> GSHMATFPELLRPLKLGRYTLRNRIIMAPLTRCQATEDGHVPRTESMLKYYEDRASAGLIIAEATMVQPNYTGFLTEPGIYSDAQIEEWRKIVDAVHKKGGLIFLQLIHAGRAGIPEKILQQPKSDQDPLAGRLLAASAIPIKDHRIPAYFAASGEKETYGVPEELTDDEVRNGIIPLFVEGAKNAIFKAGFDGVEIHGANGYLLDAFFRESSNKRQSGPYAGTTIDTRCQLIYDVTKSVCDAVGSDRVGLRISPLNGVHGMIDSNPEALTKHLCKKIEPLSLAYLHYLRGDMVNQQIGDVVAWVRGSYSGVKISN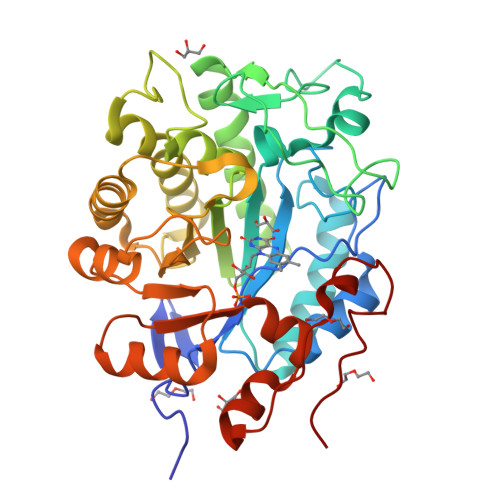LRYDFEEADQQIREGKVDAVAFGAKFIANPDLVERAQHDWPLNEPRPETYYTRTAVGYNDYPTYNK> KRFTRCGLVNELRKQGFDENLMRDWVCLVENESARYTDKIANVNKNGSRDYGLFQINDKYWCSKGSTPGKDCNVTCSQLLTDD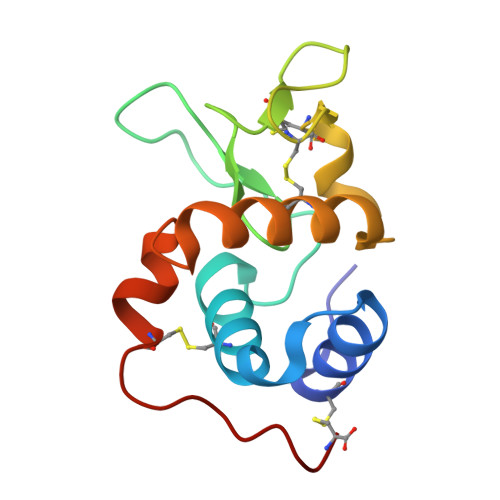ITVASTCAKKIYKRTKFDAWSGWDNHCNHSNPDISSC4-[(5-{[4-(3-CHLOROPHENYL)-3-OXOPIPERAZIN-1-YL]METHYL}-1H-IMIDAZOL-1-YL)METHYL]BENZONITRILE 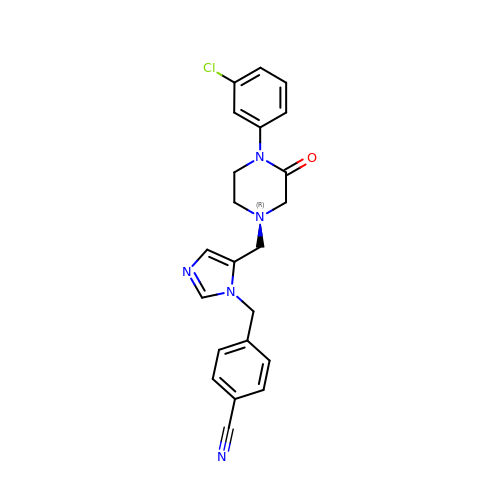| C22 H20 Cl N5 O | JNUGFGAVPBYSHF-UHFFFAOYSA-N N-[5-(5,6-dichloro-1H-indol-1-yl)pentyl]-2-sulfanylacetamide | C15 H18 Cl2 N2 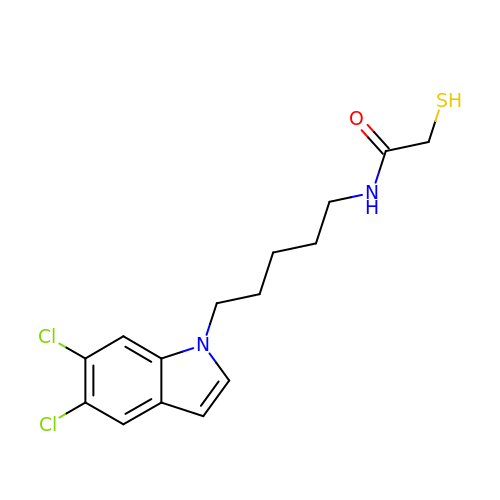O S | MHKHGVSRGWQPII-UHFFFAOYSA-N>GSMSRSKRDNNFYSVEIGDSTFTVLKRYQNLKPIGSGAQGIVCAAYDAILERNVAIKKLSRPFQNQTHAKRAYRELVLMKCVNHKNIIGLLNVFTPQKSLEEFQDVYIVMELMDANLCQVIQMELDHERMSYLLYQMLCGIKHLHSAGIIHRDLKPSNIVVKSDCTLKILDFGLARTAGTSFMMTPYVVTRYYRAPEVILGMGYKENVDIWSVGCIMGEMIKGGVLFPGTDHIDQWNKVIEQLGTPCPEFMKKLQPTVRTYVENRPKYAGYSFEKLFPDVLFPADSEHNKLKASQARDLLSKML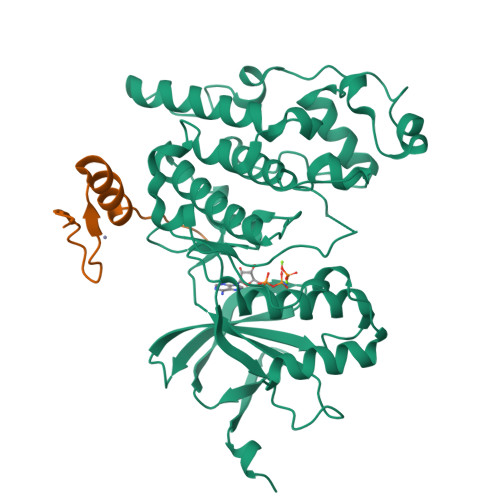VIDASKRISVDEALQHPYINVWYDPSEAEAPPPKIPDKQLDEREHTIEEWKELIYKEVMDLE[2x];>[2x]YSDDKPFLCTAPGCGRRFTNEDHLAVHKRKHEMTLKFGPA>YKIGTKALPCSECHDVFDCTGCLFEEKESSHVIPLKLNKKNPNDHKKLQKHHESLKLGDVKYYVNRGEGISGSLGTSSGNTLDDMDLINEEINKKRTNAQNATVEQTKENIFLVPLKHLRDSQFVGELLVGTPPQTVYPIFDTGSTNVWVVTTACEEESCKKVRRYDPNKSKTFRRSFIEKNLHIVFGSGSISGSVGTDTFMLGKHLVRNQTFGLVESESNNNKNGGDNIFDYISFEGIVGLGFPGMLSAGNIPFFDNLLKQNPNVDPQFSFYISPYDGKSTLIIGGISKSFYEGDIYMLPVLKESYWEVKLDELYIGKERICCDEESYVIFDTGTSYNTMPSSQMKTFLNLIHSTACTEQNYKDILKS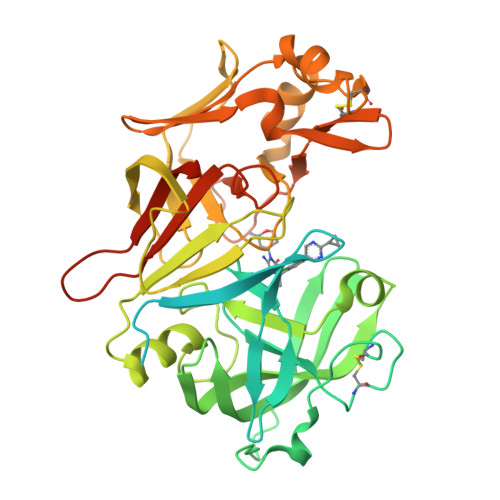YPIIKYVFGELIIELHPEEYMILNDDVCMPAYMQIDVPSERNHAYLLGSLSFMRNFFTVFVRGTESRPSMVGVARAKSKNENLYFQGSHHHHHHHH[2x]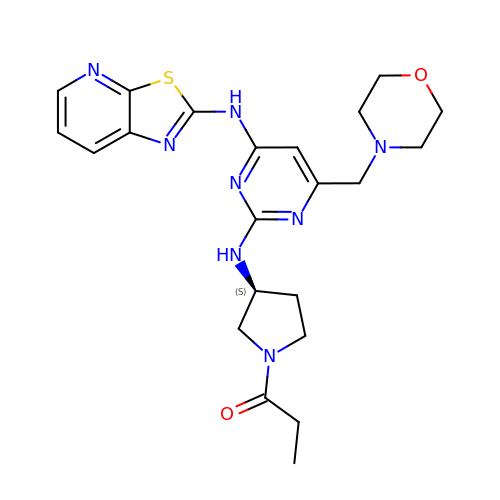1-[(3S)-3-{[4-(morpholin-4-ylmethyl)-6-([1,3]thiazolo[5,4-b]pyridin-2-ylamino)pyrimidin-2-yl]amino}pyrrolidin-1-yl]propan-1-one | C22 H28 N8 O2 S | JSHRNKDQLCOTRI-HNNXBMFYSA-N>TQEGQRYQALKAHAEEKLQLANE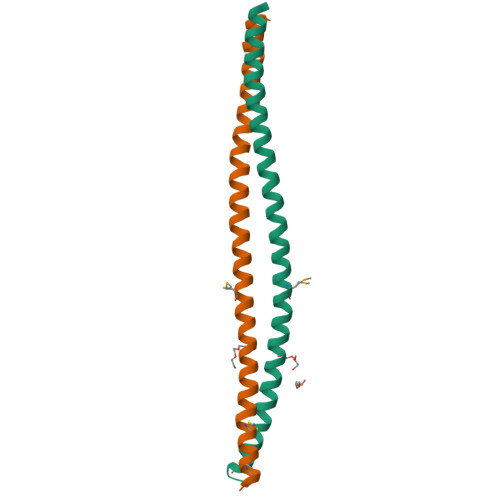EIAQVRSKAQAEALALQASLRKEQMRIQSLEKTVEQKTKENEELTRICDDLISKMEKI[8x]> XWNLVRIGL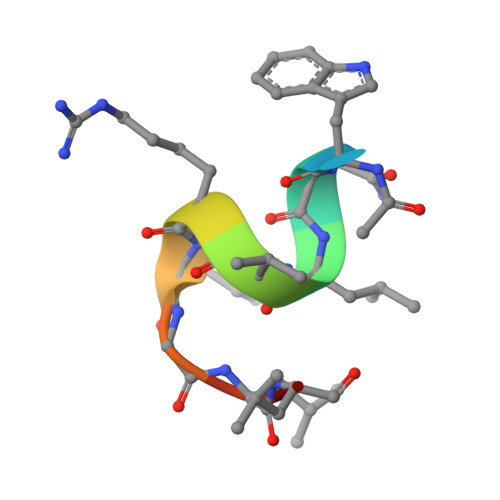LR> MGLEKTVKEKLSFEGVGIHTGEYSKLIIHPEKEGTGIRFFKNGVYIPARHEFVVHTNHSTDLGFKGQRIKTVEHILSVLHLLEITNVTIEVIGNEIPILDGSGWEFYEAIRKNILNQNREIDYFVVEEPIIVEDEGRLIKAEPSDTLEVTYEGEFKNFLGRQKFTFVEGNEEEIV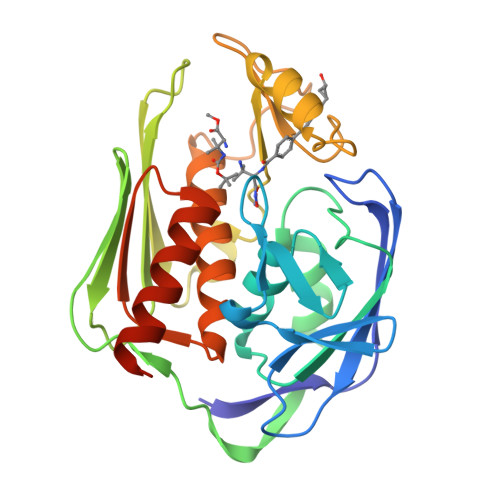LARTFAFDWEIEHIKKVGLGKGGSLKNTLVLGKDKVYNPEGLRYENEPVRHKVFDLIGDLYLLGSPVKGKFYSFRGGHSLNVKLVKELAKKQKLTRLEHHHHHH> MAPIQEYVGTLIYVGVALFIGVAALLVGALLGPKKPGRA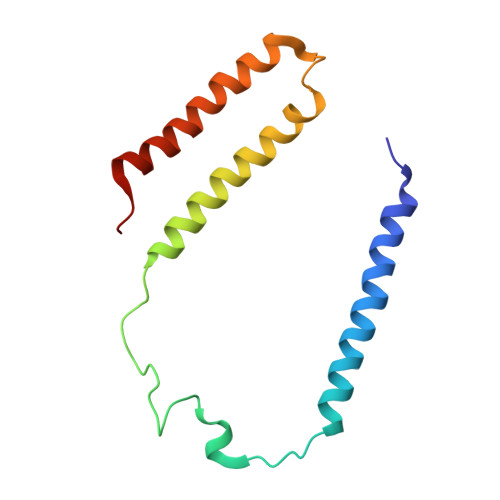KLMPYESGNDPAGEVKRFPVHFYVVAMLFILFDVEVAFLWPYAVSAGGLGLYGFLGVLAFTLLLFVGFLYEWWKGVMRWH> MTLLNDIQVWTTACAYDHLIPGRGVGVLLDDGSQVALFRLDDGSVHAVGNVDPFSGAAVMSRGIVGDRGGR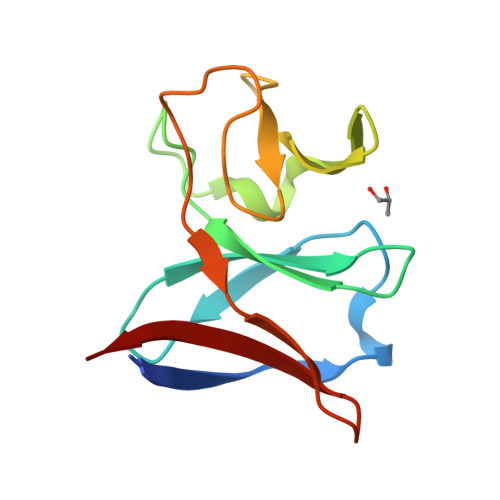AMVQSPILKQAFALDDGSCLDDPRVSVPVYPARVTPEGRIQVARVAVG> AVTYPDSVQHNETVQNLIKSLDKKNFETVLQPFSEFHNRYYKSDNGKKSSEWLQGKIQEIISASGAKGVTVEPFKHSFPQSSLIAKIPGKSDKTIVLGAHQDSINLDSPSEGRAPGADDDGSGVVTILEAFRVLLTDEKVAAGEAPNTVEFHFYAGEEGGLLGSQDIFEQYSQKSRDVKAMLQQDMTGYTKGTTDAGKPESIGIITDNVDENL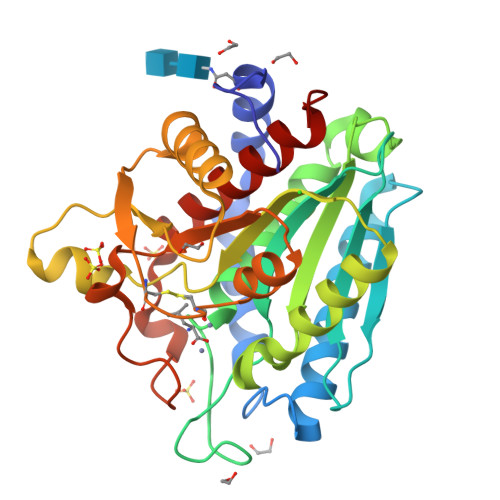TKFLKVIVDAYCTIPTVDSKCGYGCSDHASATKYGYPAAFAFESAFGDDSPYIHSADDTIETVNFDHVLQHGRLTLGFAYELAFADSL8-(4-methylsulfonylphenyl)-N-(4-morpholin-4-ylphenyl)-[1,2,4]triazolo[1,5-a]pyridin-2-amine 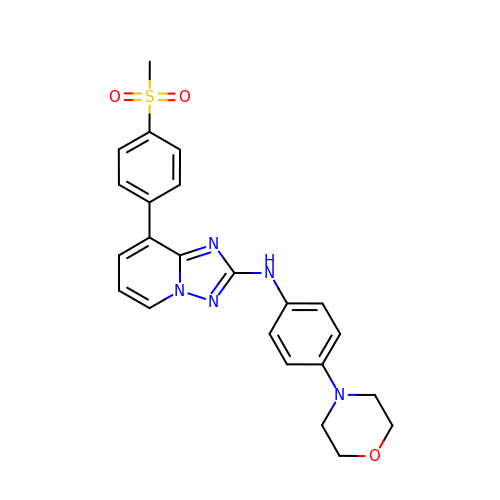| C23 H23 N5 O3 S | UUVZHZJBZYONMR-UHFFFAOYSA-N> SFYP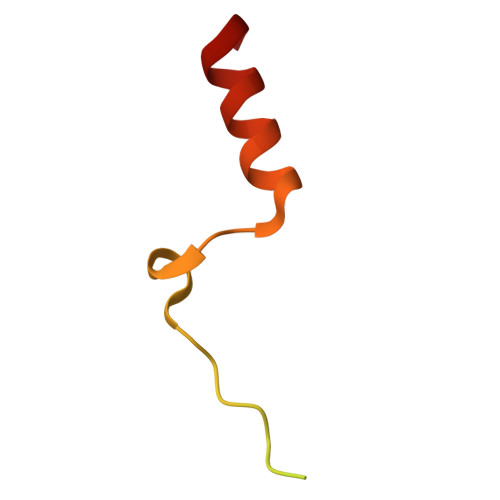DEDDFYFGGPDSTPPGEDIWKKFELLPTPPLSPSRGFAEHSSEPPSWVTEMLLENELWG> MVDAVVTVFLEKTLNILEEKGRTVSDYRKQLEDLQSELKYMQSFLKDAERQKRTNETLRTLVADLRELVYE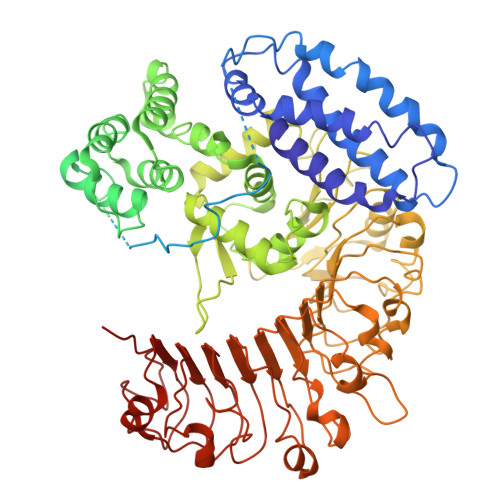AEDILVDCQLADGDDGNEQRSSNAWLSRLHPARVPLQYKKSKRLQEINERITKIKSQVEPYFEFITPSNVGRDNGTDRWSSPVYDHTQVVGLEGDKRKIKEWLFRSNDSQLLIMAFVGMGGLGKTTIAQEVFNDKEIEHRFERRIWVSVSQTFTEEQIMRSILRNLGDASVGDDIGTLLRKIQQYLLGKRYLIVMDDVWDKNLSWWDKIYQGLPRGQGGSVIVTTRSESVAKRVQARDDKTHRPELLSPDNSWLLFCNVAFAANDGTCERPELEDVGKEIVTKCKGLPLTIKAVGGLLLCKDHVYHEWRRIAEHFQDELRGNTSETDNVMSSLQLSYDELPSHLKSCILTLSLYPEDCVIPKQQLVHGWIGEGFVMWRNGRSATESGEDCFSGLTNRCLIEVVDKTYSGTIITCKIHDMVRDLVIDIAKKDSFSNPEGLNCRHLGISGNFDEKQIKVNHKLRGVVSTTKTGEVNKLNSDLAKKFTDCKYLRVLDISKSIFDAPLSEILDEIASLQHLACLSLSNTHPLIQFPRSMEDLHNLQILDASYCQNLKQLQPCIVLFKKLLVLDMTNCGSLECFPKGIGSLVKLEVLLGFKPARSNNGCKLSEVKNLTNLRKLGLSLTRGDQIEEEELDSLINLSKLMSISINCYDSYGDDLITKIDALTPPHQLHELSLQFYPGKSSPSWLSPHKLPMLRYMSICSGNLVKMQEPFWGNENTHWRIEGLMLSSLSDLDMDWEVLQQSMPYLRTVTANWCPELESFAIEDVGFRGGVWMKTPLHRT>MELYLDTASLEEIREIAAWGVLSGVTTNPTLVAKAFAAKGEALTEEAFAAHLRAICETVGGPVSAEVTALEAEAMVAEGRRLAAIHPNIVVKLPTTEEGLKACKRLSAEGIKVNMTLIFSANQALLAARAGA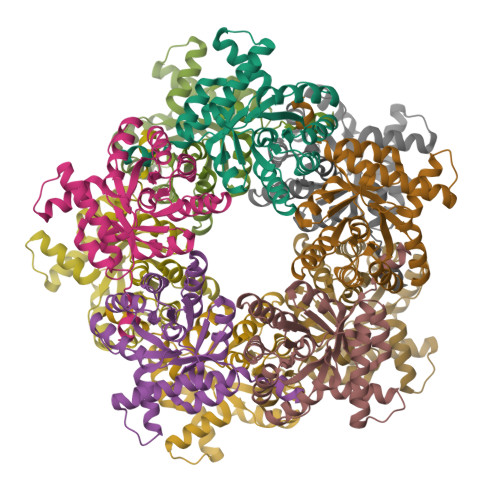SYVSPFLGRVDDISWDGGELLREIVEMIQVQDLPVKVIAASIRHPRHVTEAALLGADIATMPHAVFKQLLKHPLTDIGLKRFLEDWEKVKP[10x]>[2x]GSHMTTPSHLSDRYELGEILGFGGMSEVHLARDLRL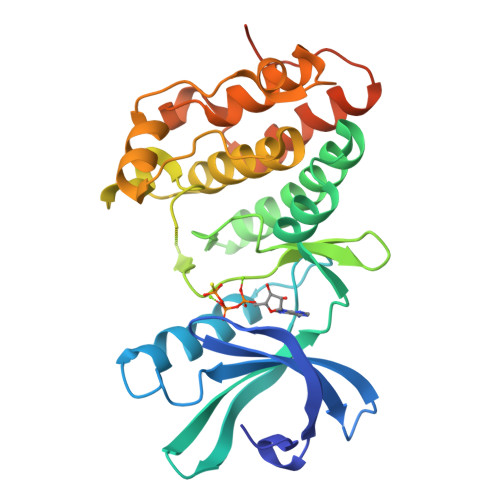HRDVAVKVLRADLARDPSFYLRFRREAQNAAALNHPAIVAVYDTGEAETPAGPLPYIVMEYVDGVTLRDIVHTEGPMTPKRAIEVIADACQALNFSHQNGIIHRDVKPANIMISATNAVKVMDFGIARAIADSGNSVTQTAAVIGTAQYLSPEQARGDSVDARSDVYSLGCVLYEVLTGEPPFTGDSPVSVAYQHVREDPIPPSARHEGLSADLDAVVLKALAKNPENRYQTAAEMRADLVRVHNGEPPEAPKVLTDAERTSLLSSAAGNLSGPR> MSDFAKVEQSLREEMTR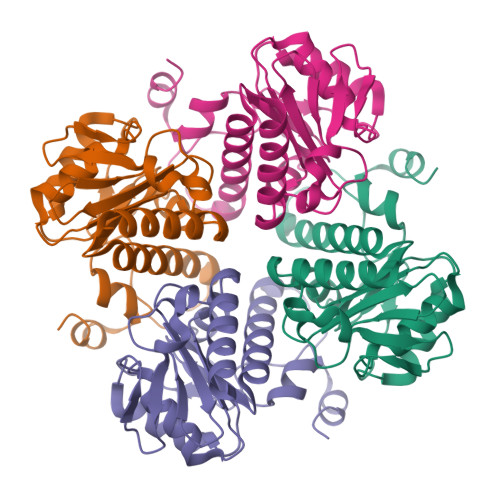IASSFFQRGYATGSAGNLSLLLPDGNLLATPTGSCLGNLDPQRLSKVAADGEWLSGDKPSAAVLFHLALYRNNPRCKAVVHLHSTWSTALSCLQGLDSSNVIRPFTPYVVMRMGNVPLVPYYRPGDKRIAQDLAELAADNQAFLLANHGPVVCGESLQEAANNMEELEETAKLIFILGDRPIRYLTAGEIAELRS>GSAMGSTSRKKVLLKVIILGDSGVGKTSLMNQYVNKKFSNQYKATIGADFLTKEVMVDDRLVTMQIWDTAGLERFQSLGVAFYRGADCCVLVFDVTAPNTFKTLDSWRDEFLIQASPRDPENFPFVVLGNKIDLENRQVATKRAQAWCYSKNNIPYFETSAKEAINVEQAFQTIARNALKQETEVELYNEFPEPIKLDKN[2x];> SAMGNSTGIKLVRKEGGLDDSVFIAVKEIGRDLYRGLPTEERIQKLEFMLDKLQNEIDQELEHNNSLVREEKETTDTRKKSLLSAALAKSGERLQALTLLMIHYRAGIEDIETLESLSLDQHSKKISKYTDDT

PDZD8 is an ER anchored lipid transfer protein containing a lipid-binding module of the synaptotagmin-like mitochondrial-lipid-binding (SMP) domain family. PDZD8 consists of an N-terminal transmembrane helix, a SMP domain, a PDZ domain, a C1 domain, and the C-terminal coiled-coil domain. PDZD8 tethers the ER to late endosomes and lysosomes by associating its C-terminal coiled-coil (CC) with the LE Rab7. The GTP-loaded Rab7A (hereafter referred to as Rab7) on the LEs recruits various effectors facilitating endosome transport along microtubule tracks and their fusion with lysosomes and autophagosomes.

The structure of the PDZD8 CC–Rab7 complex was determined at 2.1 Å resolution by molecular replacement method using a structure of the GTP-bound Rab7. In the asymmetric unit of the crystal, there were two molecules of Rab7 bound to a single molecule of the PDZD8 CC. The PDZD8 CC forms a coiled-coil structure within a single polypeptide chain and does not have intermolecular coiled-coil interaction. The three α-helices form a flat structure arranged in an α1-α3-α2 topology. Two Rab7 molecules (Rab7a-A and Rab7a-B) bind on the opposite sides of the flat CC structure and have no direct contact with each other. Two Rab7 molecules loaded with GTP have an active closed conformation of switch I and II loops. The direct recognition of the PDZD8 CC on the closed conformation of switch loops explains the GTP-dependent interaction of PDZD8 and Rab7. The MBP-PDZD8 CC bound two GTP-loaded Rab7 molecules with Kd values of 0.67 and 11.1 μM, respectively. The asymmetric bivalent binding of Rab7 and the membrane anchoring by Rab7 impose a constraint in the orientation of the PDZD8 CC–Rab7 complex, positioning the coiled-coil domain parallel to the membrane surface.>MNHKVHHHHHHIEGRHMNNSGSFSLPFKLAGLGRYVPEDIVLSSELEKKYDLPQGWCLEKQGIRERRWVKGETAAFMGAEAAKEAVRDAGLQLSDIDLIISASGSPQQAVPDGGPLVQRELGLGRSGTPAITVNASCLSFFVA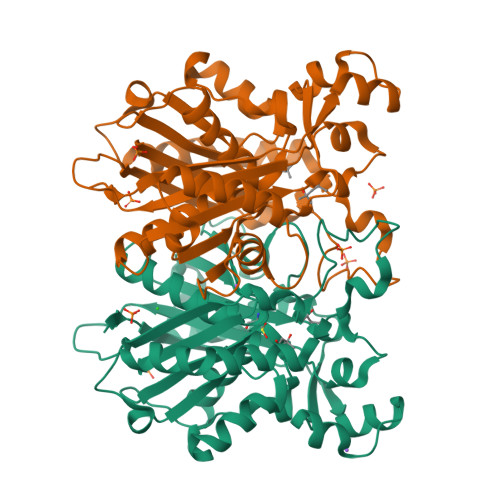LEVASNYLNMRRYRRILVVSADIASVSLDFRKPENFTLFGDAAAAAVVTLPEPGEKSCIHASHLRTYGFGAEFSEVRGGGSRKPPNSKDTRPEDNYLHMNGAELLKIGFEYLPKFTESLWKQCPDITVRDVKYIIPHQPSRVVLDYLSLSYPEEKLIRIIERFGNCIGASMPMALYEAVKLRGLQRGDKAVLTGTGSGVSFVGMVFTY[2x]> MLPNTKLHNTIFSETRKFTRESFKEIEHLTARLANDSVARHDFLFNTSIALISDYSGEDSNGNQLQATITIPNEIINPKEYDPSDYPLAEDESFFKQGHKYDYLVTFRAGSLTNTYEPKTKMYKLHAALDKLMHVRQRKSRFADLWRELCAVIASLDVWYQTTNYPLRTYVKLLFHRGDEFPFYESPSQDRIIFNDKSVASILPTFVYTCCQVGTAIMSGILTHVESIVAMNHFLHCAKDSYIDEKLKIKGIGRSWYQEALHNVGQATVPVWSQFNEVIGHRRKSTSEPHFVSSTFISLRAKRAELLYPEFNAYINRAIQLSKTQNDVANYYAACRAMTNDGTFLATLTELSLDAAVFPRIEQRLVTRPAVLMSNTRHESLKQKYTNGVGSIAQSYLSSFTDEIAKRVNGIHHDEAWLNFLTTSSPGRKLTEIEKLEVGGDVAAWSNSRIVMQAVFAREYRTPERIFKSLKAPIKLVERQQSDRRQRAISGLDNDRLFLSFMPYTIGKQIYELNDNAAQGKQAGNAFDIGEMLYWTSQRNVLLSSIDVAGMDASVTTNTKDIYNTFVLDVASKCTVPRFGPYYAKNMEVFEVGKRQSQVRYVNAAWQACALEAADSQTSTSYESEIFGQVKNAEGTYPSGRADTSTHHTVLLQGLVRGNELKRASDGKNSCLATIKILGDDIMEIFQGSESDTYDHAMSNANILNESGFATTAELSQNSIVLLQQLVVNGTFWGFADRISLWTREDTKDIGRLNLAMMELNALIDDLVFRVRRPEGLKMLGFFCGAICLRRFTLSVDNKLYDSTYNNLSKYMTLIKYDKNPDFDSTLMSLILPLAWLFMPRGGEYPAYPFERRDGTFTEDESMFTARGAYKRRLLYDVSNIREMIQQNSMALDDDLLHEYGFTGALLLIDLNILDLIDEVKKEDISPVKVSELATSLEQLGKLGEREKSRRAASDLKIRGHALSNDIVYGYGLQEKIQKSAMATKETTVQSKRVSSRLHDVIVAKTRDYKISTIPADALRLHEFEVEDVTVDLLPHAKHTSYSSLAYNMSFGSDGWFAFALLGGLDRSANLLRLDVASIRGNYHKFSYDDPVFK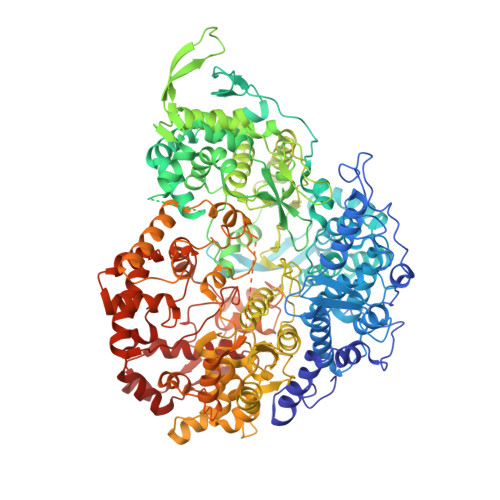QGYKIYKSDATLLNDFFTAISAGPKEQGILLRAFAYYSLYGNVEYHYVLSPRQLFFLSDNPVSAERLVRIPPKYYVSTQCRALYNIFSYLHILRSIANNWGKRLKMVLHPGLIAYVRGTSQGAILPEADNV>[2x]MTRTLPPGVSDERFDAALQRFRDVVGDKWVLSTADELEAFRDPYPVGAAEANLPSAVVSPESTEQVQDIVRIANEYGIPLSPVSTGKNNGYGGAAPRLSGSVIVKTGERMNRILEVNEKYGYALLEPGVTYFDLYEYLQSHDSGLMLDCPDLGWGSVVGNTLDRGVGYTPYGDHFMWQTGLEVVLPQGEVMRTGMGALPGSDAWQLFPYGFGPFPDGMFTQSNLGIVTKMGIALMQRPPASQSFLITFDKEEDLEQIVDIMLPLRINMAPLQNVPVLRNIFMDAAAVSKRTEWFDGDGPMPAEAIERMKKDLDLGFWNFYGTLYGPPPLIEMYYGMIKEAFGKIPGARFFTHEERDDRGGHVLQDRHKINNGIPSLDELQLLDWVPNGGHIGFSPVSAPDGREAMKQFEMVRNRANEYNKDYAAQFIIGLREMHHVCLFIYDTAIPEAREEILQMTKVLVREAAEAGYGEYRTHNALMDDVMATFNWGDGALLKFHEKIKDALDPNGIIAPGKSGIWSQRFRGQNL

Among them, one gene codes for a eugenol oxidase (EUGO) that displays significant sequence identity with VAO (≈40 %) and a similar but not fully overlapping pattern of substrate preferences. In addition to the oxidation of vanillyl alcohol and the hydroxylation of eugenol, EUGO can efficiently catalyze the dehydrogenation of various phenolic ketones and the selective oxidation of a racemic secondary alcohol—4‐(1‐hydroxyethyl)‐2‐methoxyphenol. The overall structure of EUGO is highly similar to that of VAO, as indicated by a 1.1 Å rmsd for 490 Cα atom pairs (45 % sequence identity). As predicted, EUGO also shares with VAO the presence of a characteristic covalent bond between His390 (equivalent to His422 of VAO) and the C8M atom of the flavin ring.

Incubation of eugenol (1) with the enzyme in Tris⋅HCl buffer (pH 8.0) containing 1 % (v/v) DMSO afforded coniferyl alcohol (2) with complete conversion after 4 h at room temperature. The structural bases of substrate and inhibitor binding by the cavity were explored by solving the crystal structures of EUGO in complexes with isoeugenol (inhibitor), coniferyl alcohol (2, reaction product and inhibitor), and vanillin (4, reaction product); these were obtained by crystal soaking, resulting in highly defined electron density maps. All these ligands bind with their aromatic moiety stacking against the pyrimidine ring of the flavin and the Cα atom of the aliphatic substituent lying right above the flavin N5 atom at a distance of 3.2 Å. In this orientation, the ligand 4‐hydroxy group is H‐bonded to Tyr91 and Tyr471 and is also in close contact with Arg472 (3.5 Å). These three residues are involved in the stabilization of the phenolate form of the substrate and are strictly conserved in VAO. Collectively, these features are fully consistent with the substrate being bound in the phenolic form and oxidized through a reaction mechanism involving a hydride transfer from the Cα to the flavin N5, coupled to the stabilization of a p‐quinone methide intermediate as demonstrated for VAO.> SH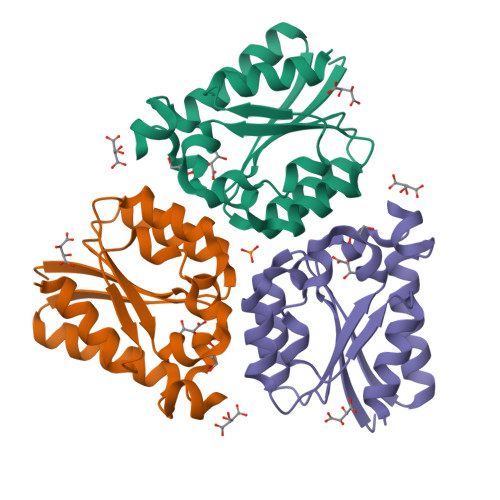MKILVINGPNLNFLGIREKNIYGNENYEYLVNMINEYCKSKNIEVECYQSNHEGAIIDKIQEAYFNGTDGIVINPGAYTHYSYAIRDALASVSHIKKIEVHISNVNEREEFRHISVTEPVCNGQIVGQGLKGYIMAIDMLNS> UGUG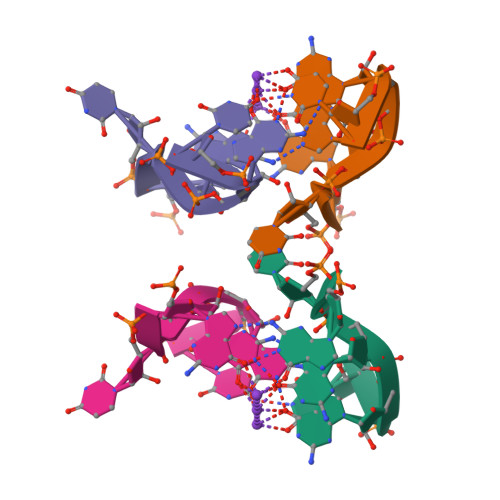GU>ASVSRLLGFDSIPAATTDTISLPKGYKSSVLISWGQPLHKNGPAFDPSGNGTAAAQEVQFGDNNDGMSLFEFPGEKNRALMAINNEYTNYRYLYPHGGMPQSAEDVRKALACEGVSVIEVQRKNGQWQFVQGSRYNRRIHGNSPLRISGPAAGHELMKTSADKHGKKVLGTFQNCANGKTPWGTYLTCEENFTDCFGSSNAQQQFDPAQKRYGVSAASREI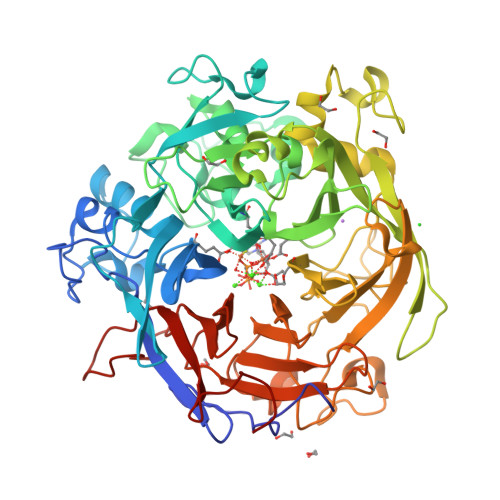NWHPFDPRFDMAKNPNELNRHGWVVEIDPFDPQSTPVKRTALGRFKHENAALAETDDGRAVVYMGDDERGEFIYKFVSRDKINHRNAKANRDILDHGTLYVARFDAGDGNPDHPKGQGQWIELTHGKNGIDASSGFADQAEVLIHARLAASVVGATRMDRPEWIVVSPKDGQVYCTLTNNAKRGEDGQPVGGPNPREKNVYGQILRWRTDRDDHASKTFAWDLFVVAGNPSVHAGTPKGGSSNITPQNMFNSPDGLGFDKAGRLWILTDGDSSNAGDFAGMGNNQMLCADPATGEIRRFMVGPIGCEVTGISFSPDQKTLFVGIQHPGENGGSTFPEHLPNGKPRSSVMAITREDGGIVGAHHHHHH[2x]> KEVVLLDFAAAGGELGWLTHPYGKGWDLMQNIMNDMPIYMYSVCNVMSGDQDNWLRTNWVYRGEAERIFIELKFTVRDCNSFPGGASSCKETFNLYYAESDLDYGTNFQKRLFTKIDTIAPDEITVSSDFEARHVKLNVEERSVGPLTRKGFYLAFQDIGACVALLSVRVYYKKCPELLQGLAHFPETIAGSDAPSLATVAGTCVDHAVVPPGGEEPRMHCAVDGEWLVPIGQCLCQAGYEKVEDACQACSPGFFKFEASESPCLECPEHTLPSPEGATSCECEEGFFRAPQDPASMPC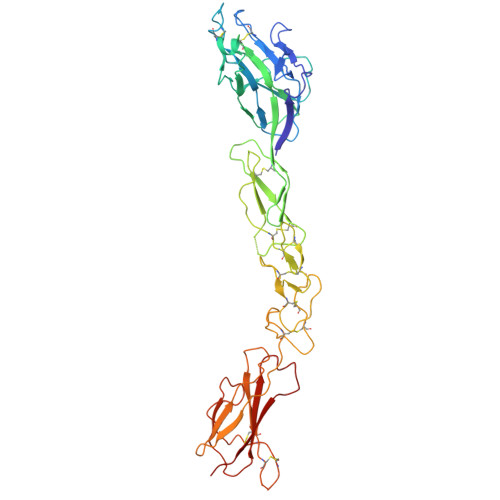TRPPSAPHYLTAVGMGAKVELRWTPPQDSGGREDIVYSVTCEQCWPESGECGPCEASVRYSEPPHGLTRTSVTVSDLEPHMNYTFTVEARNGVSGLVTSRSFRTASVSIN Vadadustat | C14 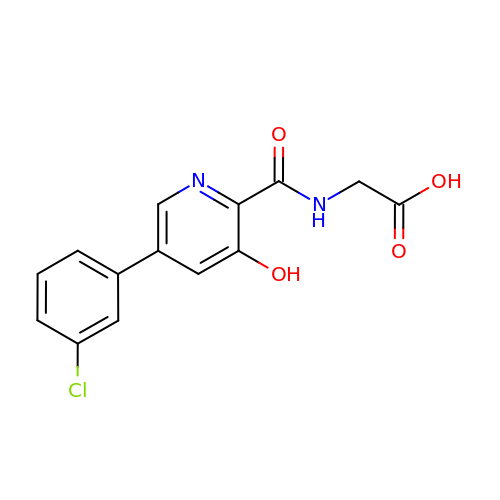H11 Cl N2 O4 | JGRXMPYUTJLTKT-UHFFFAOYSA-N>[2x]MDREALLQAVKEARELAKPRNFTQSFEFI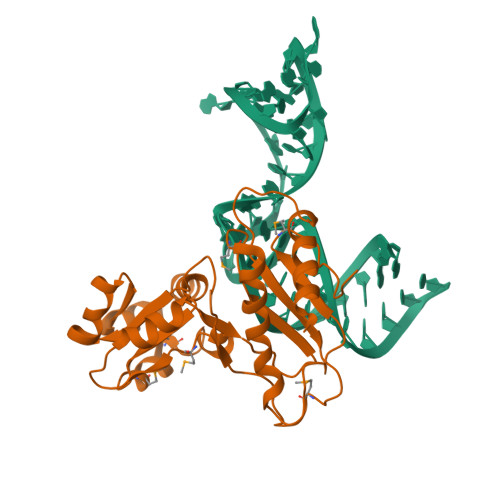ATLKEIDMRKPENRIKTEVVLPHGRGKEAKIAVIGTGDLAKQAEELGLTVIRKEEIEELGKNKRKLRKIAKAHDFFIAQADLMPLIGRYMGVILGPRGKMPKPVPANANIKPLVERLKKTVVINTRDKPYFQVLVGNEKMTDEQIVDNIEAVLNVVAKKYEKGLYHIKDAYVKLTMGPAVKVKKEKAKKK Within this class of proteins, the bromodomain and extraterminal domain (BET) family contains four members that are transcriptional coregulators and that recognize acetyllysines (AcKs) using a tandem pair of highly homologous bromodomains (BDs). Despite heavy academic and industry investment in this area, the generation of paralog-selective inhibitors has proved elusive because of the extremely high sequence similarity between the bromodomains of family members (90 to 95% within the acetyllysine-binding pocket residues). Using the highly conserved BET BDs as a model system, we conducted three mRNA display-based RaPID (random nonstandard peptides integrated discovery) screens using a single library (which contains >1012 unique members). Crystal structures of 13 distinct peptide–bromodomain complexes revealed highly diverse structures and binding modes among the cyclic peptide ligands.

We also solved structures of another lariat-type peptide, 4.2C, bound to a BD1 and a BD2 domain. In contrast, 4.2B and 4.2C are members of smaller families that are detected only in the BRD4-BD2 selection. In line with this observation, 4.2B and 4.2C showed significant selectivity for BD2 domains over BD1 domains. The peptide is helical and bivalent, recruiting two molecules of BRD2-BD2. Its “primary” interaction has the 4.2C helix binding in the same location as the other helical peptides but its long axis is ∼30° offset from that of the others. The second interaction is also mediated by an AcK–pocket interaction but with the helix unusually oriented “end on” to the pocket. No interaction was detected with any non-BET BD and, within the BET family, binding was only observed to the BD2s of BRD2 and BRD4, consistent with our SPR data. Finally, a NOESY of peptide 4.2C, which adopts an α-helical structure when bound, displays several amide–amide NOEs, indicating helical propensity in the sequence. However, the relatively small number of medium- and long-range NOEs suggests that the peptide exhibits significant conformational dynamics rather than a single well-defined conformation.

>SSEQLKHCNGILKELLSKKHAAYAWPFYKPVDASALGLHDYHDIIKHPMDLSTVKRKMENRDYRDAQEFAADVRLMFSNCYKYNPPDHDVVAMARKLQDVFEFRYAKMP[8x];>[4x]XWKGYLCLRKRIQ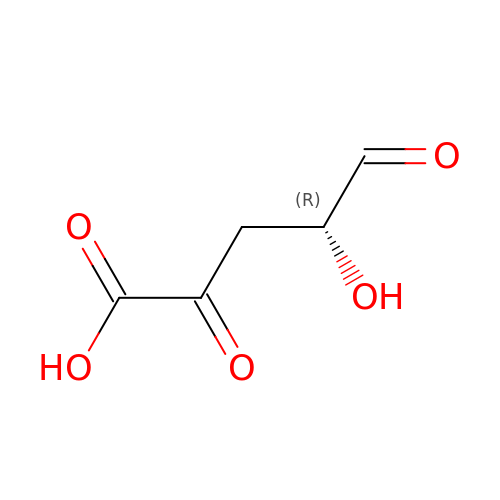(4R)-4-hydroxy-2,5-dioxopentanoic acid | C5 H6 O5 | QZKCWTOLHHFWCD-GSVOUGTGSA-N> XQARSDIEKLKEAIRDTNKAVQSVQSSIGNLIVAIKSVQDYVNKEIVPSIARX;> XVALDPFDFSIVLN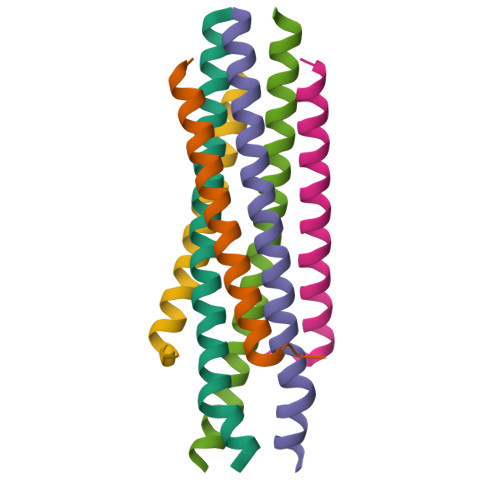KIKSQLEESKEWIRRSNKILDSIX> MKQVCVLGNGQLGRMLRQAGEPLGIAVWPVGLDAEPAAVPFQQSVITAEIERWPETALTRQLARHPAFVNRDVFPIIADRLTQKQLFDKLHLPTAPWQLLAERSEWPAVFDRLGELAIVKRRTGGYDGRGQWRLRANETEQLPAECYGECIVEQGINFSGEVSLVGARGFDGSTVFYPLTHNLHQDGILRTSVAFPQANAQQQARAEEMLSAIMQELGYVGVMAMECFVTPQGLLINELAPRVHNSGHWTQNGASISQFELHLRAITDLPLPQPVVNNPSVMINLIGSDVNYDWLKLPLVH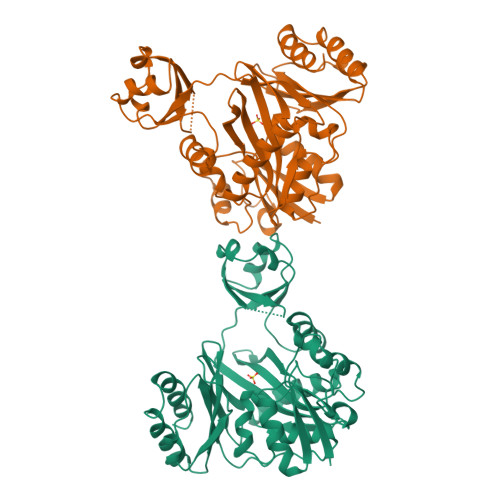LHWYDKEVRPGRKVGHLNLTDSDTSRLTATLEALIPLLPPEYASGVIWAQSKFG>[2x]MRVLVTGGSGYIGSHTCVQLLQNGHDVIILDNLCNSKRSVLPVIERLGGKHPTFVEGDIRNEALMTEILHDHAIDTVIHFAGLKAVGESVQKPLEYYDNNVNGTLRLISAMRAANVKNFIFSSSATVYGDQPKIPYVESFPTGTPQSPYGKSKLMVEQILTDLQKAQPDWSIALLRYFNPVGAHPSGDMGEDPQGIPNNLMPYIAQVAVGRRDSLAIFGNDYPTEDGTGVRDYIHVMD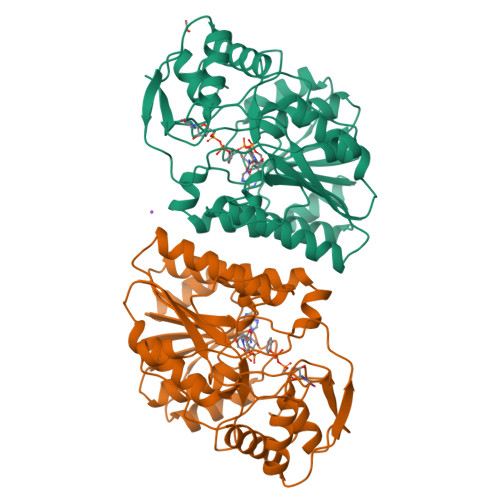LADGHVVAMEKLANKPGVHIYNLGAGVGNSVLDVVNAFSKACGKPVNYHFAPRREGDLPAYWADASKADRELNWRVTRTLDEMAQDTWHWQSRHPQGYPD>[2x]GCGGGAA;>U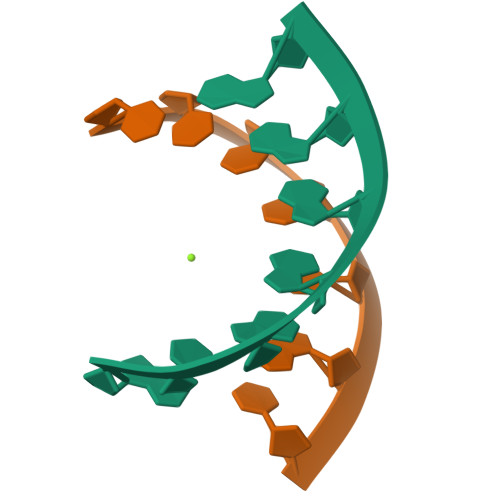UCCCGC[2x]>[2x]REVLTGGHSVSAPQENRIYVMDSVFMHLTESRVHVYDYTNGKFLGMVPTAFNGHVQVSNDGK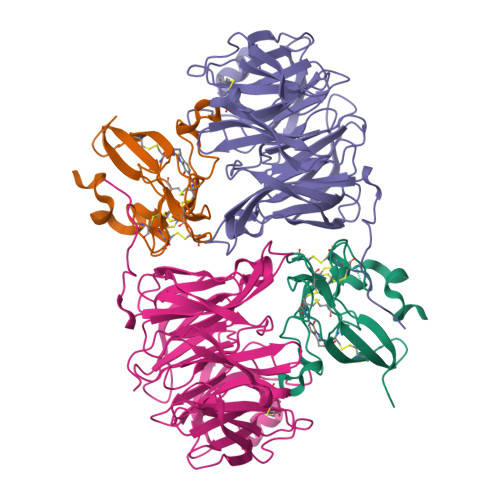KIYTMTTYHERITRGKRSDVVEVWDADKLTFEKEISLPPKRVQGLNYDGLFRQTTDGKFIVLQNASPATSIGIVDVAKGDYVEDVTAAAGCWSVIPQPNRPRSFMTICGDGGLLTINLGEDGKVASQSRSKQMFSVADDPIFIAPALDKDKAHFVSYYGNVYSADFSGDEVKVDGPWSLLNDEDKAKNWVPGGYNLVGLHRASGRMYVFMHPDGKEGTHKFPAAEIWVMDTKTKQRVARIPGRDALSMTIDQQRNLMLTLDGGNVNVYDISQPEPKLLRTIEGAAEASLQVQFHPVGGT;>[2x]HISLNPDLANEDEVNSCDYWRHCAVDGFLCSCCGGTTTTCPPGSTPSPISWIGTCHNPHDGKDYLISYHDCCGKTACGRCQCNTQTRERPGYEFFLHNDVNWCMANENSTFHCTTSVLVGLAKN> RVTTVGDLAVLEGRSVMIPCHYGPQYASYVKYWCRGSVKDLCTSLVRSDAPRGPAAAGEDKVVMFDDPVQQVFTVTMTELQKEDSGWYWCGVEVGGVWSADVTASLHINVIQGLSVVNSMVSGEEGTSVTVQCLYSQGYRQHEKRWCRSGDWSSCLVTDGEGRYEDQAVEIRDDLTKAFTVTLKGLARRDTGWYWCAAGQQQVAVYILVTPPSHHHHHH

Protection is conferred largely through the function of the polymeric Immunoglobulin receptor (pIgR), which transports and stabilizes secretory antibodies and also functions as an innate immune factor. The transport cycle of pIgR starts when pIgR at the basolateral membrane binds dIgA or pIgM, and the resulting complex is transcytosed to the apical surface where proteases cleave the pIgR ectodomain (now referred to as secretory component, SC), releasing it into the mucosa as a complex with dIgA or pIgM. SC specifically protects secretory Ig from proteolytic degradation and confers innate recognition functions upon SIgA and SIgM, allowing them to bind and exclude bacteria. Here we report the first crystal structures of intact SC proteins, comparing the highly-evolved five-domain human SC (hSC) and a two-domain teleost fish SC (tSC), a relative of the first vertebrate SC ancestor.

To compare SC structures across evolution and to facilitate the design of chimeric proteins for characterizing SC-ligand interactions, we solved the 1.7Å crystal structure of teleost fish SC (tSC) (Rcryst = 18.5%; Rfree = 21.5%). Teleost fish express the oldest recognizable pIgR protein, which transports polymeric versions of IgM and IgT/IgZ (a teleost Ig specialized in mucosal immunity) to the mucosa. In addition, tSC contains just two extracellular domains, tD1 and tD2. tD1 and tD2 share homology with mammalian D1 and D5, respectively, but CDR loop residues implicated in mammalian SC interactions with pIg are not conserved. The structure of tSC revealed two tandem Ig-like domains related by ~90°. Like hSC domains D1 and D3-D5, tSC domains are IgSF folds that include the canonical B to F strand disulfide bond and a second disulfide bond linking the C and C’ strands. tD1 and tD2 share a similar topology, but only 72 of 97 Cα atoms could be aligned (rmsd = 0.87Å). Aligning fish and human SC domains resulted in rmsds of 0.77Å for tD1 and D1 (83 of 100 Cα atoms) and 1.08Å for tD2 and D5 (64 of 97 Cα atoms). The largest structural differences between tSC and hSC domains are in regions between the C’ and D strands, where tD1 residues at positions similar to the C” strand are disordered and the tD2 C” strand hydrogen bonds to the D strand on the A-B-E-D face rather than to the C’ strand on the A’-G-F-C face, similar to other IgSF proteins such as IREMs (immune receptors expressed on myeloid cells). In contrast to the human D1 CDR1 α-helical turn, both tSC CDR1 loops include a 310 helical turn and are structurally similar to human D5 CDR1. The interface between the two tSC domains is formed by residues in the tD1 A’-B and E-F loops and residues in tD2 CDR1 and DE loop, burying a total surface area of 591Å2. Ten of the 17 residues in the interface are well conserved among representative fish species, and five inter-domain hydrogen bonds may limit inter-domain flexibility.> FNLSSHSPEASVHL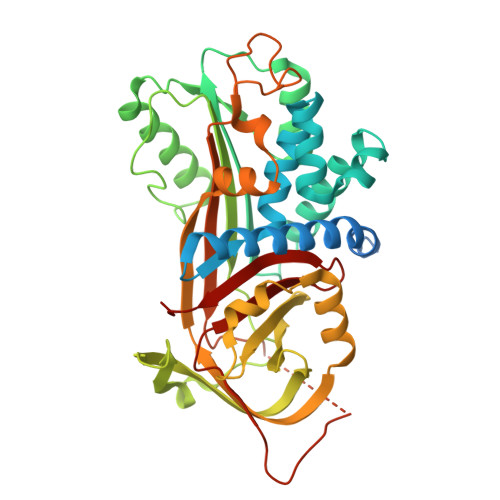ESQDYENQTWEEYTRTDPREEEEEEEEKEEGKDEEYWLRASQQLSNETSSFGFNLLRKISMRHDGNVIFSPFGLSVAMVNLMLGTKGETKVQIENGLNLQALSQAGPLILPALFKKVKETFSSNRDLGLSQGSFAFIHKDFDIKETYFNLSKKYFDIEYVSINFQNSSQARGLINHCIVKETEGKIPKLFDEINPETKLILVDYVLFKGKWLTPFDPSFTEADTFHLDKYRAIKVPMMYREGNFTSTFDKKFRCHILKLPYQGNATMLVVLMEKTGDYLALEDYLTVDLVETWLQNMKTRKMEVFFPKFKLNQRYEMHELLKQMGIRRLFSTSADLSELSAMARNLQVSRVLQQSVLEVDERGTEAVSGTLSEIIAYSMPPAIKVNRPFHFIIYEEMSRMLLFLGRVVNPTVL>[4x]SASIPDIKLSSGHLMPSIGFGCWKLANATAGEQVYQAIKAGYRLFDGAEDYGNEKEVGDGVKRAIDEGLVKREEIFLTSKLWNNYHDPKNVETALNKTLADLKVDYVDLFLIHFPIAFKFVPIEEKYPPGFYCGDGNNFVYEDVPILETWKALEKLVAAGKIKSIGVSNFPGALLLDLLR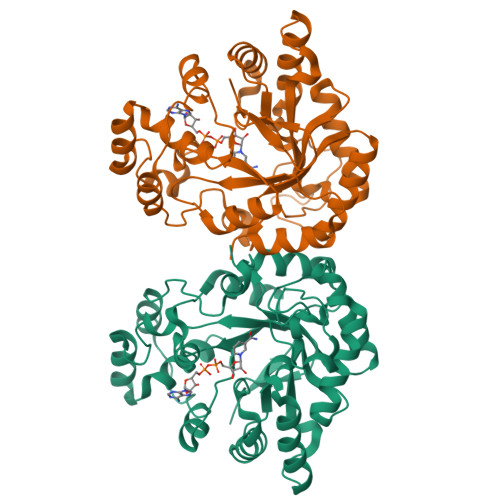GATIKPAVLQVEHHPYLQQPKLIEFAQKAGVTITAYSSFGPQSFVEMNQGRALNTPTLFAHDTIKAIAAKYNKTPAEVLLRWAAQRGIAVIPKSNLPERLVQNRSFNTFDLTKEDFEEIAKLDIGLRFDDPWDWDNIPIFV> MVGLADVAVLYSGGKDSNYALYWAIKNRFSVKFLVTMVSENEESYMYHTINANLTDLQARALGIPLVKGFTQGEKEKEVEDLKRVLSGLKIQGIVAGALASKYQRKRIEKVAKELGLEVYTPAWGR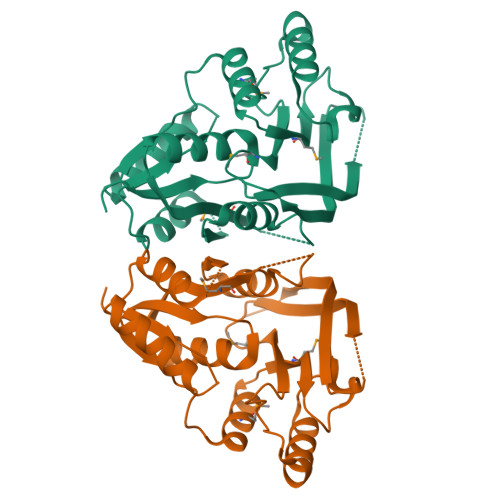DAKEYMRELLNLGFKIMVVGVSAYGLDESWLGRILDESALEELITLNEKYKVHVAGEGGEFETFVLDMPLFKYKIVVDKAKKVWEPCTSSGKLIIEEAHLESKLEHHHHHH Alginate is produced by a synthase-dependent exopolysaccharide secretion system—a conserved molecular mechanism in Gram-negative bacteria for manufacturing and exporting carbohydrate polymers, including cellulose, acetylated cellulose, poly-ß-d-N-acetylglucosamine (PNAG), Pel, and alginate. Synthase-dependent systems are characterized by a membrane-embedded glycosyl transferase involved in polymer synthesis, a cyclic-di-GMP binding protein that regulates polymer synthesis, one or more periplasmic polymer-modifying enzymes, an outer membrane-linked protein with a tetratricopeptide repeat (TPR)-containing domain, and a ß-barrel porin through which the polymer is exported. In this study, we focus on the alginate proteins AlgX and AlgK involved in polymer acetylation and export, respectively. The AlgKX protein complex reveals the molecular details of a crucial protein–protein interaction involved in alginate production and provides fundamental insight into how a polymer modification enzyme and export protein function collaboratively in synthase-dependent secretion systems.

To understand how AlgK and AlgX interact at a molecular level, we co-crystallized Pseudomonas putida AlgK without its native signal sequence (AlgKPp33–484) and full-length P. putida AlgX (AlgXPp1–479) and determined the structure of the AlgKXPp complex to 2.5 Å resolution. The AlgKXPp complex crystallized in space group I 4 2 2 with a single copy of AlgKPp and AlgXPp in the asymmetric unit. In the AlgKXPp complex, we were able to model eight TPR motifs (R3-R10) in AlgKPp (residues 138–452) and residues 29–468 of AlgXPp. The N-terminus of AlgXPp (residues 29–37) adopts an extended conformation in the complexed structure that could not be modeled in the isolated AlgXPa structure, suggesting that the extended N-terminus of AlgX may be disordered and dynamic in nature, thus requiring interaction with AlgK for stabilization. The AlgKXPp structure reveals that it’s mainly the N-terminus of AlgXPp (residues 30–37) that interacts with TPRs R9-R10 of AlgKPp, however additional residues outside the N-terminus of AlgXPp also interact with AlgKPp. PISA also calculated the interaction interface to have a buried surface area of 1015 Å2 mediated by 12 hydrogen bonds and one salt bridge. The side chains of AlgXPp E35 and AlgKPp R404 form a salt bridge, while the main chains of these residues interact via hydrogen bonding. To understand how specificity might be conferred, we next examined the surface hydrophobicity of AlgKXPp, AlgKXPa, and AlgKXPs. This analysis revealed a highly conserved, hydrophobic patch on the N-terminus of AlgX that is buried in a conserved, deep hydrophobic groove on AlgK. Examining the surface electrostatic properties of AlgKXPp, we discovered an electropositive region spanning 44 Å across the surface of AlgKXPp that extends from the active site of AlgXPp to the concave surface of AlgKPp, from R9 towards the N-terminus.

> MTPHLMKLLGLSAALLAISQGVRAEDVKAPTFSAEPCCQLCPEAHDASRYTTRYQQNFTTLVQAQGDWLFRTREDLRTEFNTTPAGYKRLQQVHDAFKKRGVELVVVYQPTRGLVNRNMLNPAEKAAFDYQKALGNYQAMLKRFASMGYNVPDLSPLTNEQLAAADQGKDFYFRGDQHWTPYGAERAAKIVADTVHKMPAFEGIPRKEFETRKSGRMGKTGTLHNVAGQLCGTSYAVQYMDQFATEPKGASGGDDLFGDSGNAQITLVGTSHSGKNYNFSGFLEQYIGADVLNVAFPGGGLEGSMIQYLGSEEFQKNPPKILIWEFSPLYRLDQETIWRQILGLLDDGCDDRPALMSASTTLKPGKNELMVNGKGGVIKDLINRNLQMDVKFEDPSVKVLQATLWYLNGRHEDIKLEKPETSDTDGRFVFQMREDEDWASQRLLAFEVQGPESGTQKVEAKLCKRNNFAVPAQTAQAGQLEHHHHHH;> MCAGLPDQRLANEALKRGDTALAERNYKALADLGYSEAQVGLADIKVATRDPSQIKEAEATYRAAAATSPRAQARLGRLLVAKPDSTQAEREEAETLLKQAAKQGQSNTLIPLAMLYLSYPQSFPKVNAQQQIDQWRAAGNPEAGLAQVLLYRTQGTYDQHLGEVEKICKAALNTTDICYVELATVYQKRGQADQQAALLGQLKSAYARGAVPATRVDSVARVLADRSLGQTDEKTAKELLEQVAPANPASWVSLAQLVYDFPELGDTDQLMAYIDKGREAEQPRAELLLGRLYYEGKTLPADAQKAEQHLQAAAEAGEISAHYYLGQLYRRGYLGNVEPQKAVDHLLAAARGGQNSADYALAQLFSEGHGIRPQPGNAWVFAQLSQANPTPQSAELLQQLDQQLTPDQRNQAQQLLDQEKRARGSLAQGANSTLALEALQDDEKEVDGEDSLLEHHHHHH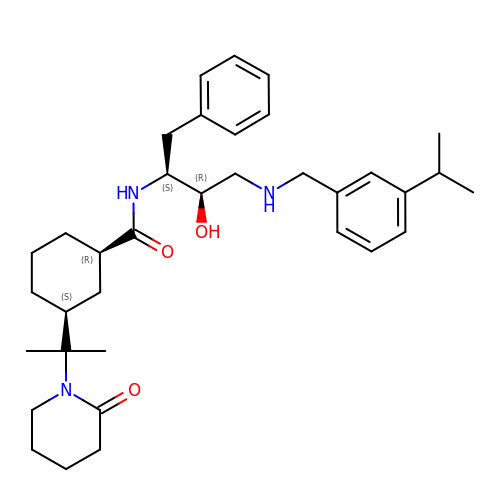(1R,3S)-N-[(1S,2R)-1-benzyl-2-hydroxy-3-{[3-(1-methylethyl)benzyl]amino}propyl]-3-[1-methyl-1-(2-oxopiperidin-1-yl)ethyl]cyclohexanecarboxamide | C35 H51 N3 O3 | MFPZDLDVZIAMTN-OKDNLZPVSA-N GH19 chitinase hydrolyzes the glycosidic bonds of chitin, namely beta-1, 4-linked N-acetyl-D-glucosamine. One of the physiological roles of chitinase is to defend plants against pathogenic fungi by degrading chitin, a major component of the cell wall of many fungi. By revealing the evolutionary history and loops appearance of GH19 chitinase, we discover that one loop which is remote from the catalytic site, is necessary to acquire the new antifungal activity. We demonstrate that this remote loop directly accesses the fungal cell wall, and surprisingly, it needs to adopt a defined structure supported by long-range intramolecular interactions to perform its function.

After we confirmed that the tree topology did not change based on the presence/absence of loop regions in the MSA, we used the tree based on the unmodified MSA and selected five ancestral nodes where InDels of the loop regions occurred, designated Anc1 to Anc5 based on the presence/absence of loop regions in the extant sequences. To get structural insights into the emergence of antifungal activity in GH19 chitinase, we first solved the X-ray crystal structure of Anc4 and Anc5. Crystal structures of Anc4 and Anc5 solved to 1.13 Å and 1.57 Å, respectively. Overall, the backbone structures of Anc4 and Anc5 were nearly identical (RMSD of Cα = 0.478 Å) and the orientation of catalytic residues is similar, suggesting that loop I and II addition/removal did not cause major structural disruptions. All five ancestral proteins showed a similar level of chitinase activity to the two modern GH19 chitinases, while Anc5 also exhibited antifungal activity. Insertion of loop I to Anc4 resulted in a loss of catalytic activity of Anc4. The loss of the hydrolytic activity in Anc4 via loop I insertion might be due to the lack of disulfide bonding between loop I and the core scaffold. However, it is worth noting that the addition of loop II to Anc4 did not improve its antifungal activity. Anc4 and 5 differ by 45 substitutions, suggesting that loop II enhances antifungal activity in combination with residues in the protein scaffold. By fluorescence microscope experiments, we observed that only Anc5 and Anc5ΔLoop I bound to the surface of fungal hyphae. This result is consistent with the result that Anc5 and Anc5ΔLoop I showed 28-fold stronger antifungal activity than Anc4, suggesting that the acquisition of loop II is necessary to access the substrate in the cell wall of fungi to perform antifungal activity.

> MVSRSMFDQLFPNRNSFYTYDAFIAAAKSFPSFGTTGDTDVRKREIAAFFAHVSHETSGLVYIEEINQSNDYCDPSTQYPCAPGKQYYGRGPLQLSWNYNYGPCGDALGLDLLNNPDLVAQDPVIAFKTALWFWMTPQSPKPSCHDVMTGNWTPSSADLAAGRVPGFGVTTNIINGGLECGKGNPAQAENRVNYYKDFCNQLGVSPGSNLDCANMRPFG>[4x]GSHMEQRILKFLEELGEGKATTAHDLSGKLGTPKKEINRVLYSLAKKGKLQKEAGT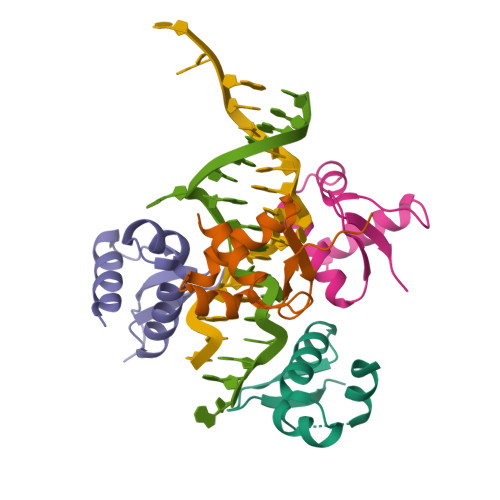PPLWKIAVSTQ> AAAAVVTYLGAANVVGAANGTVTAN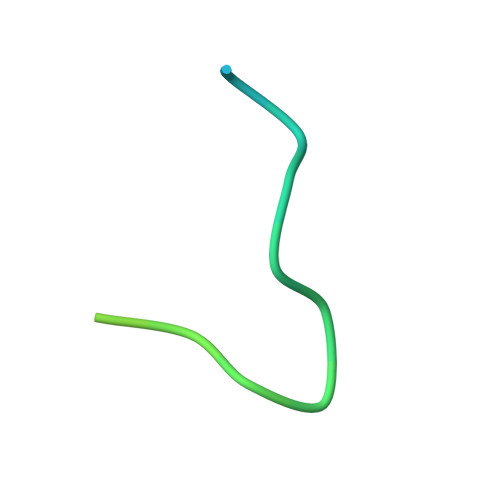AVANTNAVA> STRSPRPFNEIPSPGDNGWLNLYHFWRETGTHKVHLHHVQNFQKYGPIYREKLGNVESVYVIDPEDVALLFKSEGPNPERFLIPPWVAYHQYYQRPIGVLLKKSAAWKKDRVALNQEVMAPEATKNFLPLLDAVSRDFVSVLHRRIKKAGSGNYSGDISDDLFRFAFESITNVIFGERQGMLEEVVNPEAQRFIDAIYQMFHTSVPMLNLPPDLFRLFRTKTWKDHVAAW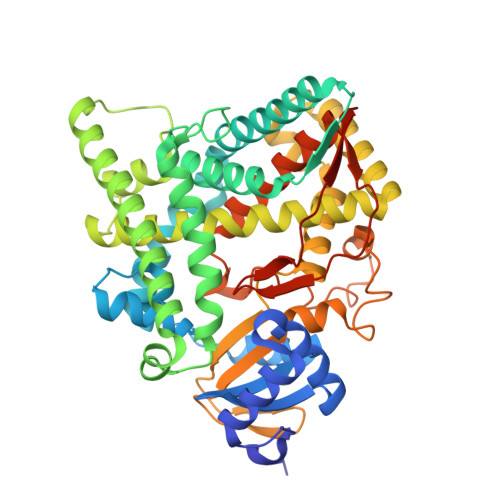DVIFSKADIYTQNFYWELRQKGSVHHDYRGILYRLLGDSKMSFEDIKANVTEMLAGGVDTTSMTLQWHLYEMARNLKVQDMLRAEVLAARHQAQGDMATMLQLVPLLKASIKETLRLHPISVTLQRYLVNDLVLRDYMIPAKTLVQVAIYALGREPTFFFDPENFDPTRWLSKDKNITYFRNLGFGWGVRQCLGRRIAELEMTIFLINMLENFRVEIQHLSDVGTTFNLILMPEKPISFTFWPFNQEATQQHHHHHH> VLNGYWGYQEFLDEFPEQRNLTNALSEAVRAQPVPLSKPTQRPIKISVVYPGQQVSDYWVRNIASFEKRLYKLNINYQLNQVFTRPNADIKQQSLSLMEALKSKSDYLIFTLDTTRHRKFVEHVLDSTNTKLILQNITTPVREWDKHQPFLYVGFDHAEGSRELATEFGKFFPKHTYYSVLYFSEGYISDVRGDTFIHQVNRDNNFELQSAYYTKATKQSGYDAAKASLAKHPDVDFIYACSTDVALGAVDALAELGREDIMINGWGGGSAELDAI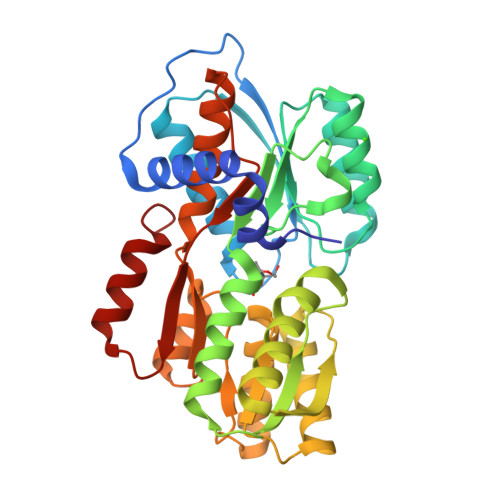QKGDLDITVMRMNDDTGIAMAEAIKWDLEDKPVPTVYSGDFEIVTKADSPERIEALKKRAFRYSDN>[2x]RILPDSVDWREKGCVTEVKYQ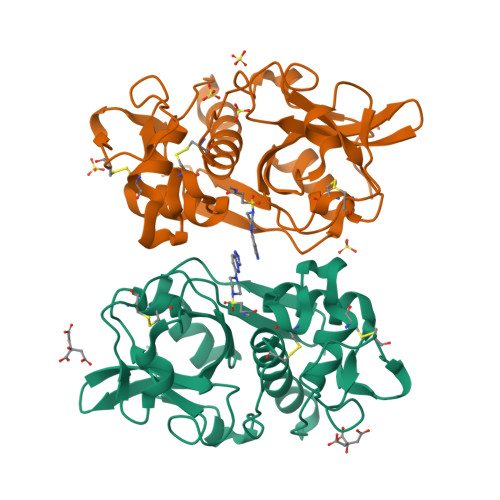GSCGACWAFSAVGALEAQLKLKTGKLVSLSAQNLVDCSTEKYGNKGCNGGFMTTAFQYIIDNKGIDSDASYPYKAMDQKCQYDSKYRAATCSKYTELPYGREDVLKEAVANKGPVSVGVDARHPSFFLYRSGVYYEPSCTQNVNHGVLVVGYGDLNGKEYWLVKNSWGHNFGEEGYIRMARNKGNHCGIASFPSYPEIHHHHHH>HSFLSPDAQVLVLAISSHPLPTLAAFLASRRDELLRADITSLLKALELSGHWEWALALLRWAGKEGAADASALEMVVRALGREGQHDAVCALLDETPLPPGSRLDVRAYTTVLHALSRAGRYERALELFAELRRQGVAPTLVTYNVVLDVYGRMGRSWPRIVALLDEMRAAGVEPDGFTASTVIAACSRDGLVDEAVAFFEDLKARGHAPCVVTYNALLQVFGKAGNYTEALRVLGEMEQNGCQPDAVTYNELAGTYARAGFFEEAARCLDTMASKGLLPNAFTYNTVMTAYGNVGKVDEALALFDQMKKTGFVPNVNTYNLVLGMLGKKSRFTVMLEMLGEMSRSGCTPNRVTWNTMLAVSGKRGMEDYVTRVLEGMRSSGVELSRDTYNTLIAAYGRCGSRTNAFKMYNEMTSAGFTPCITTYNALLNVLSRQGDWSTAQSIVSKMRTKGFKPNEQSYSLLLQCYAKGGNVAGIAAIENEVYGSGAVFPSWVILRTLVIANFKCRRLDGMETAFQEVKARGYNPDLVIFNSMLSIYAKNGMYSKATEVFDSIKRSGLSPDLITYNSLMDMYAKCSESWEAEKILNQLKCSQTMKPDVVSYNTVI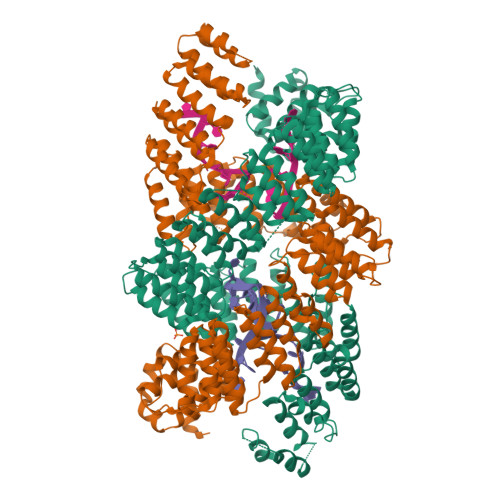NGFCKQGLVKEAQRVLSEMVADGMAPCAVTYHTLVGGYSSLEMFSEAREVIGYMVQHGLKPMELTYRRVVESYCRAKRFEEARGFLSEVSETDLDFDKKALEAYIEDAQFGR[2x]>MFIKPGRCPKPAVQEDFDAARYLGVWYDIQRLPNKAQKGECATATYSLSPGVGFSVFNRERLANGTIKSVIGSAIAEDPCEPAKLQFFHENAAPVPYWVLSTDYDNYALVY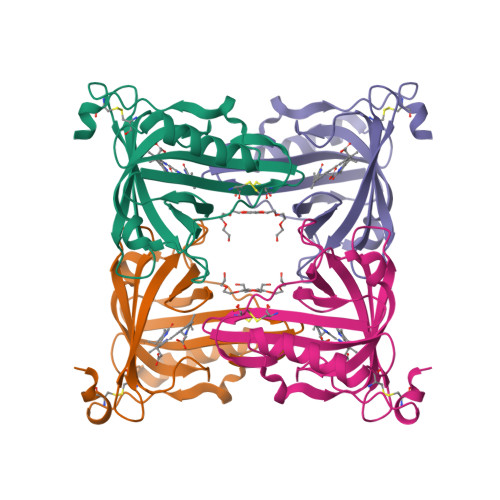SCINLGASHAAYASIVSRQPTLPEETIKKLQGTMSSFGVGVDTLLTTNQDAAYCSAMNQKLAAALEHHHHHH[2x]>MGSSHHHHHHSQDPNSISTTMSSYSIQQSQKMLTQLQIDYATNTSSNTVVAYLHNVGETTISYLQNSVVYFGPNGQLQPVGYNSGSSPYWTVTSNSLQPGSVVKIIIYLSSPLSSNQYYTIQIVTPNGY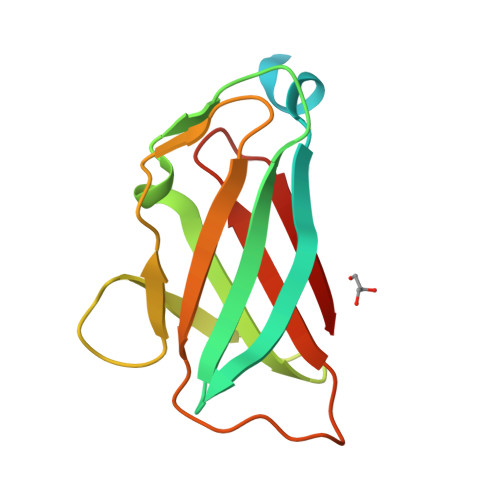TVSYMF[2x]> AEHYNLISWNVNGLRAAVKKGFLDLLLEHRFDIVCVQETKVSQDKLPREVKNIQGYYNYFVSAEQNGYSGVGTFSKNKPIKLEKGMGIEVFDREGR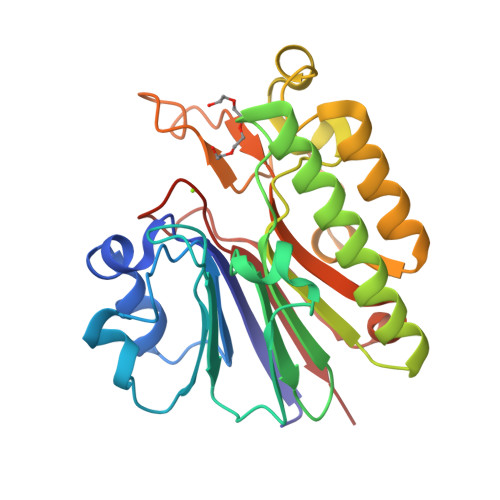FLRTDYEDFVLLNIYFPNGKMSQERLGYKMAFYDAFLDYANALKSEGKKLVICGDVNTAHKEIDLARPKQNEMISGFLPEERAWMDKFLAAGYLDSFRMFNPEGGNYSWWSYRTGARSRNVGWRLDYVFVSENLRENVKSASIYPEIMGSDHCPVGLELEFV> HHMDVPADSHIKYEDAIDYWTDVDATVDGVLGGYGEGTVVPTMDVLGSNNFLRKLKSRMLPQENNVKYAVDIGAGIGRVSKTMLHKHAAKIDLVEPVKPFIEQMHVELAELKDKGQIGQIYEVGMQDWTPDAGKYWLIWCQW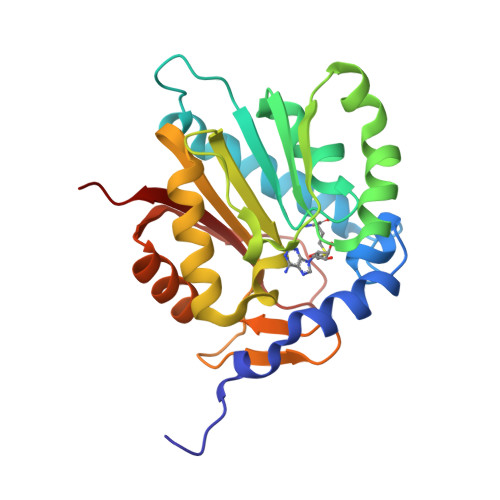CVGHLPDAELVAFLKRCIVGLQPNGTIVVKENNTPTDTDDFDETDSSVTRSDAKFRQIFEEAGLKLIASERQRGLPRELYPVRMYALKPMPN>[5x]MFSGIKGPNPSDLKGPELRILIVHARGNLQAIEPLVKGAVETMIEKHDVKLENIDIESVPGSWELPQGIRASIARNTYDAVIGI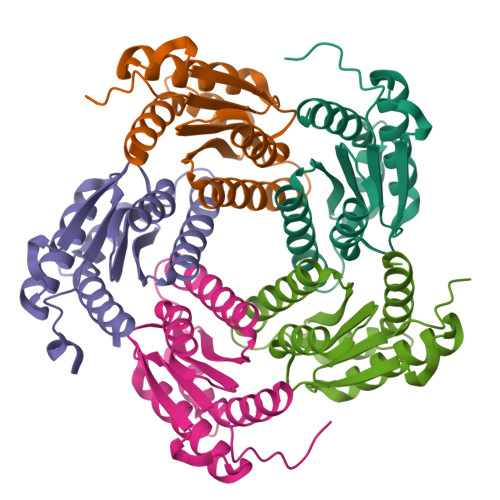GVLIKGSTMHFEYISEAVVHGLMRVGLDSGVPVILGLLTVLNEEQALYRAGLNGGHNHGNDWGSAAVEMGLKALY>SLFELGKMILQETGKNPAKSYGAYGCNCGVLGRGKPKDATDRCCYVHKCCYKKLTGCNPKKDRYSYSWKDKTIVCGENNPCLKELCECDKAVAICLRENLGTYN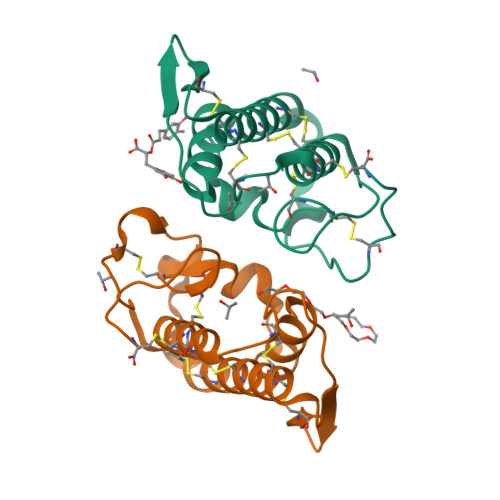KLYRYHLKPFCKKADDC[2x]> VRVSIERLWSQYFEARAKLGSLEPDEREAAETLEKRVRGLKDRLVVNYSPLVKYAAGRVTARSTGAVDQEEILSWGILGLLDAVETFDAGKGAKFETYAISKIKWAIL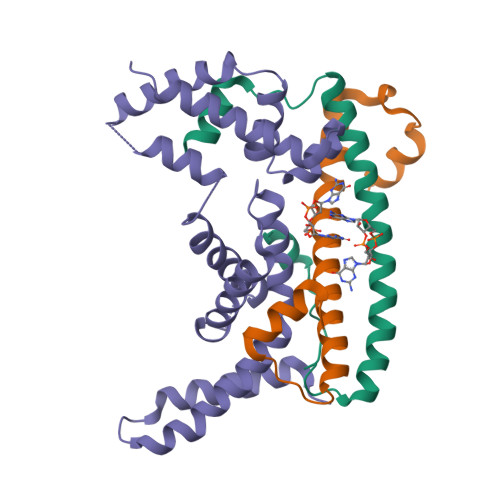DELRRLDXXXXXXXXXXXEAAEIEELRRNLVEAIKNLAERERLVTTFYFYEGLTLREIGKALGLTEGRISQILRQSLGKLRDSLSEPRTS;>MGEETYEGTSGREGGRHEEEVETRAARESAEEVWGGTEDLTSLSVEELKGLLARFDEEEKRISYRRRVIQGRIDVIRAEIVRRGGAVLSPEELARVLMGDVGDESEGGASGDRRGDGA[2x]> EFMAIERTLSIVKPDAVSKNHIGEIFARFEKAGLKIVATKMKHLSQADAEGFYAEHKERGFFGDLVAFMTSGPVVVSVLEGENAVL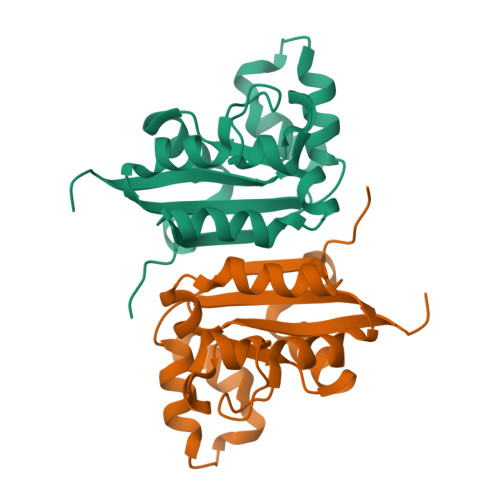AHREILGATNPKEAAPGTIRADFAVSIDENAAHGSDSVASAEREIAYFFADNEICPRTR Here, we determine the high-resolution structures of cyclic di-pyrimidine-synthesizing cGAS/DncV-like nucleotidyltransferases (CD-NTases) in clade E (CdnE) in its apo, substrate-, and intermediate-bound states. CD-NTases share an N-terminal core domain with templated and non-templated polymerases of the nucleotidyltransferase (NTase) superfamily, but the C-terminal helical domain shows a higher degree of variation. Three conserved acidic residues in the central β-sheet of the NTase domain coordinate with two metal ions (A and B) that are essential for catalysis. Based on sequence conservation and structural similarity, it is proposed that the cyclic di-pyrimidine-synthesizing CdnE proteins, including ClCdnE, EfCdnE, and LpCdnE, form smaller donor pockets that act as molecular gauges to recognize and retain the binding of pyrimidine nucleotides but weaken or exclude the binding to purine nucleotides.

By including substrate UTP or UMPnPP and cofactor MgCl2 in the crystallization solutions, we obtained the complex crystals of ClCdnE-UTP, LpCdnE-UTP, and LpCdnE-UMPnPP and refined them to 2.6-Å, 1.95-Å and 2.2-Å resolution, respectively. In the LpCdnE-UTP complex crystal, similar binding modes of the donor and acceptor nucleotides to the active site were observed for both protein molecules. In addition to the Mg-B ion, the α-phosphate of the donor UTP also forms a coordinate bond with a Mg ion, Mg-A, which further shares the Asp67 side-chain and a water molecule with Mg-B in octahedral-complex formation. The other ligands are the Asp139 side-chain, the ribose O3’ of the acceptor nucleotide, and a water molecule. The γ-phosphate group of the donor formed four hydrogen bonds with Ser53, Asn59, Lys201, and Ser220 of the protein in LpCdnE, showing remarkably stronger interactions than those in ClCdnE and EfCdnE. Besides the bond of O3’ to Mg-A, the acceptor ribose has O2’ hydrogen bonded to the Asp67 side-chain. LpCdnE binds more strongly to the acceptor triphosphate than ClCdnE. Although there is some disorder in the β- and γ-phosphate groups, the triphosphate is with hydrogen bond to the backbone N of Asp124, Lys125, and Ala126 in the βC–βD loop, and salt bridged to the Lys125 side-chain. Instead, Trp277 and Trp276 form extensive hydrophobic contacts with the base moiety of donor UTP/UMPnPP in the substrate-bound ClCdnE and LpCdnE, respectively. In LpCdnE, the Glu262 and Gln274 side chains also come together to form a hydrogen bond and restrict the donor-binding site for pyrimidine nucleotides.

>MSIDWEQTFRKWSKPSSETESTKAENAERMIKAAINSSQILSTKDISVFPQGSYRNNTNVREDSDVDICVCLNTLVLSDYSLVPGMNDKLAELRTASYTYKQFKSDLETALKNKFGTLGVSRGDKAFDVHANSYRVDADVVPAIQGRLYYDKNHNAFIRGTCIKPDSGGTIYNWPEQNYSNGVNKNKSTGNRFKLIVRAIKRLRNHLAEKGYNTAKPIPSYLMECLVYIVPDQYFTGDSYKTNVENCINYLYNQIDSSDWTEINEIKYLFGSHQMWNKTQVKEFLLTAWSYIQKNLEHHHHHH[2x]>[2x]SNAMN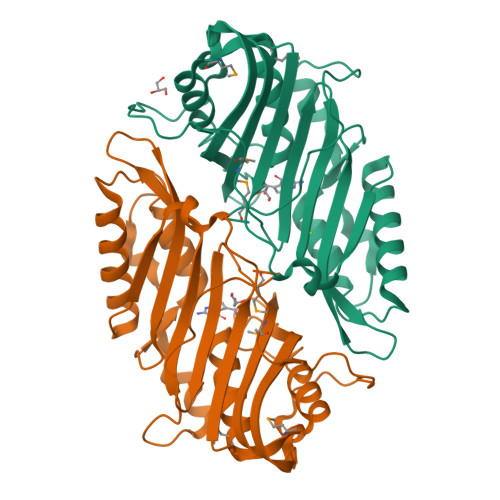RLKNMSKYSDAKELASLTLGKKTEYANQYDPSLLQPVPRSLNRNDLHLSATLPFQGCDIWTLYELSWLNQKGLPQVAIGEVSIPATSANLIESKSFKLYLNSYNQTRFASWDEVQTRLVHDLSACAGETVTVNVKSLNEYTAEPIVTMQGECIDDQDIEIANYEFDDALLQGAAQGEEVSEVLHSHLLKSNCLITNQPDWGSVEIAYHGAKMNREALLRYLVSFREHNEFAEQCVERIFTDIMRYCQPQSLTVYARYTRRGGLDINPFRSSHQSAPNHNQRMARQ TERTIARY-BUTYL ALCOHOL | C4 H10 O | 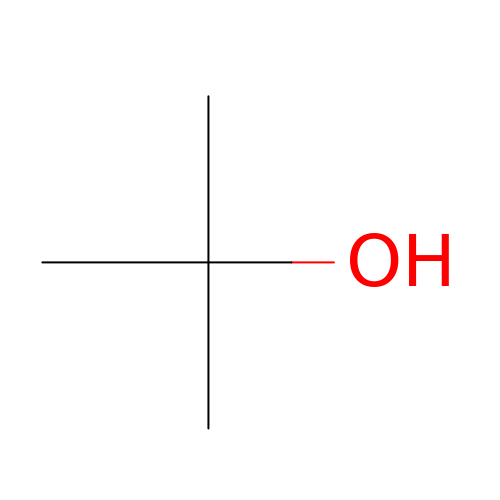DKGAVHZHDRPRBM-UHFFFAOYSA-N>[2x]SHMTAVTLDGGWRVRLVPGQEQG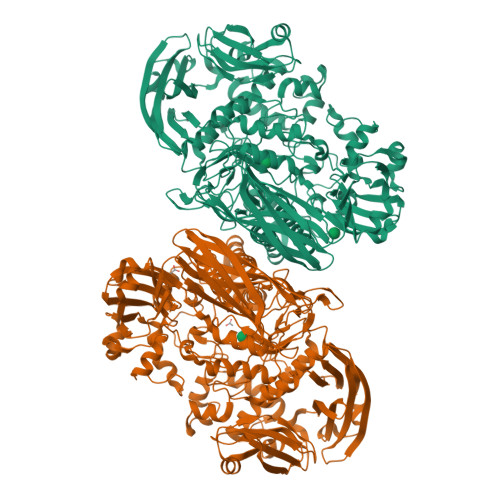KTYPKAAAWLPAQVPGAVQTDLIAAKIVPDPFYRDNEGKIQWAGLSDWQYQTRFTVDAATLKREHVELVFDGLDTFAEVTLNGKQLLSADNMFRQWRVDAKSLLKRGDNLLEVKLYSPIKKIQPWLAKQPYALPGAYDSAFGDEPEARHSSTYVRKAPYNFGWDWGPRMVNAGIWKDVRVEAWDAVRVDGLHIAQQRVDAHSAQVQAQLDLQAGRSGPVQVTLDVLGPDGQKVGQFTQDAVVDPGQNRVDLAVRIANPKRWFPAGYGAQDRYTFVASVRDADGDSQQIKRVTGLRSVELRREKDRFGKSMEIVINGIPIFAKGANLIPLDAFPARVTHERMRSTLQDARDANMNMLRMWGGGHYQDDYFYDVADELGIMIWQDFMFGGAVPPYDVEFRENTRQEAIEQVKRLRDHPSLVLWCGNNEVQTGWENWGDRVKFKQSVDPEERTRIERGMTTLFGTVFREVVATYDSDVPYWATSPGTDFDGAADQTNDGDMHYWKVWGGPALPVTEYLNVTPRFMSEYGLQSFPDMRTVRAFAEPGDMDPESPVMRVHQKFDKGNGNKRLMLYIRREFGEPKDFESFVYLSQLMQAEGINIAASHLRASRPQSMGSLYWQLNDVWPGASWSSVDYYGRWKALHYHARRFYAPEMIAALRNDKGQTEVSLVSDRTTPLTARWRMRVMGMDGKVLSKREEKASVNALSSQHVGNFSDKQLLGSADPKRTYAVFELLDGDTLLSREVVFFAPAKQLALPAAKIDSQWRADGDGYALTLTSDTLAREVWLSFGDVDATLSDNAFDLLPGEPLTVRVTSKAALAQLQSALQVRDLAATLAGAPPEP(3~{R},6~{R})-6-[(2~{S})-butan-2-yl]-3-(2,3-dihydro-1~{H}-inden-2-yl)-1-[(1~{R})-1-(2-methyl-1,3-oxazol-4-yl)-2-morpholin-4-yl-2-oxidanylidene-ethyl]piperazine-2,5-dione | C27 H34 N4 O5 | 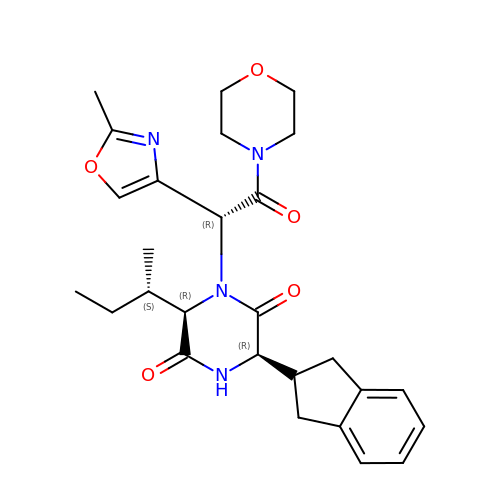PLVGDGRBPMVYPB-FDUHJNRSSA-N(R)-2-(3-ADAMANTAN-1-YL-UREIDO)-3-(3-CARBAMIMIDOYL-PHENYL)-N-PHENETHYL-PROPIONAMIDE | C29 H37 N5 O2 | 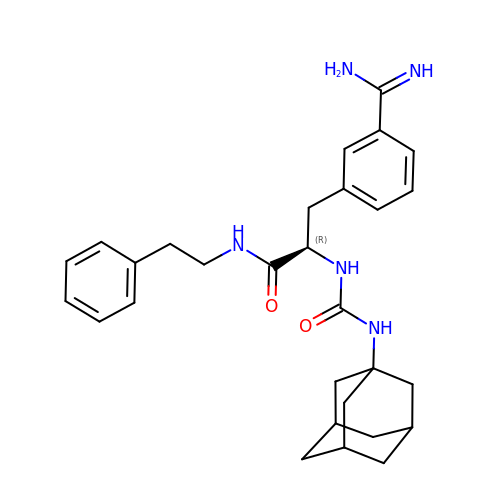QYKLXCYULDLMPX-ZEFMGYOLSA-N>[2x]ARFSIEGKSLKLDAITTEDEKSVFAVLLEDDSVKEIVLSGNTIGTEAARWLSENIASKKDLEIAEFSDIFTG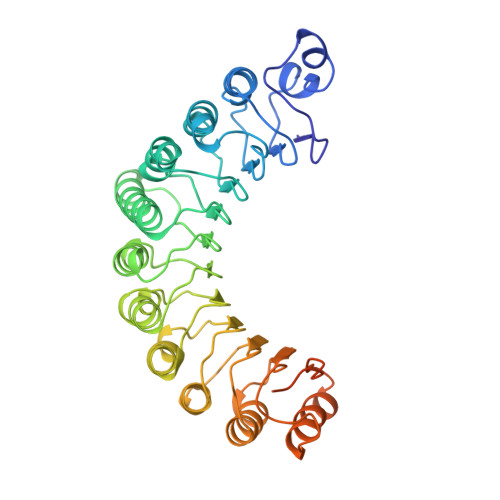RVKDEIPEALRLLLQALLKCPKLHTVRLSDNAFGPTAQEPLIDFLSKHTPLEHLYLHNNGLGPQAGAKIARALQELAVNKKAKNAPPLRSIICGRNRLENGSMKEWAKTFQSHRLLHTVKMVQNGIRPEGIEHLLLEGLAYCQELKVLDLQDNTFTHLGSSALAIALKSWPNLRELGLNDCLLSARGAAAVVDAFSKLENIGLQTLRLQYNEIELDAVRTLKTVIDEKMPDLLFLELNGNRFSEEDDVVDEIREVFSTRGRGELDELDDMEELTDEEEEDEEEEAESQSPEPETSEEEKEDKELADELSKAHI> ATKHFTLKSDVLFNFNKATLKPEGQQALDQLYTQLSNMDPKDGSAVVLGYTDRIGSEAYNQQLSEKRAQSVVDYLVAKGIPAGKISARGMGESNPVTGN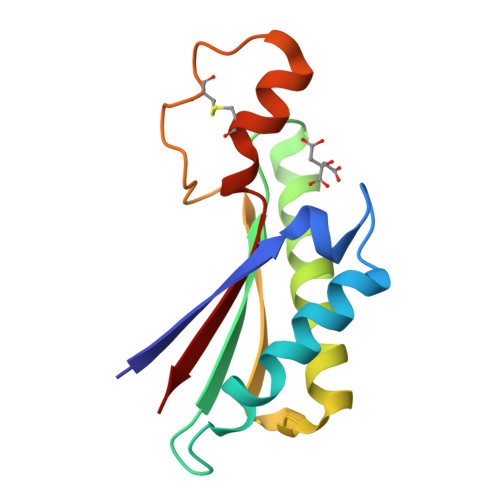TCDNVKARAALIDCLAPDRRVEIEVKG> MAMRQCAIYGKGGIGKSTTTQNLVAALAEMGKKVMIVGCDPKADSTRLILHSKAQNTIMEMAAEAGTVEDLELEDVLKAGYGGVKCVESGGPEPGVGCAGRGVITAINFLEEEGAYEDDLDFVFYDVLGDVVCGGFAMPIRENKAQEIYIVCSGEMMAMYAANNISKGIVKYANSGSVRLGGLICNSRNTDREDELIIALANKLGTQMIHFVPRDNVVQRAEIRRMTVIEYDPKAKQADEYRALARKV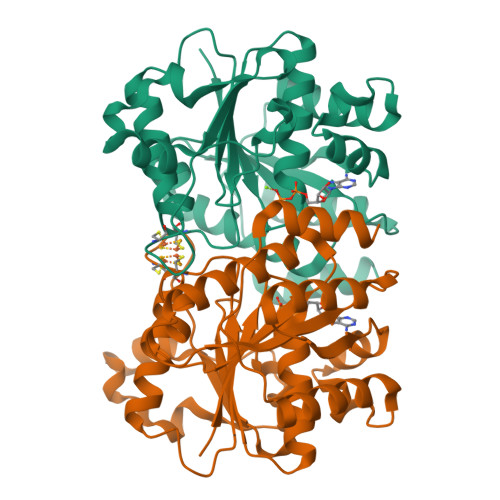VDNKLLVIPNPITMDELEELLMEFGIMEVEDESIVGKTAEEV The cysteine desulfurase IscS is a highly conserved master enzyme initiating sulfur transfer via persulfide to a range of acceptor proteins involved in Fe-S cluster assembly, tRNA modifications, and sulfur-containing cofactor biosynthesis. IscS is a highly conserved, widely distributed pyridoxal-5′-phosphate (PLP)-dependent enzyme, with 60% sequence identity between the enzyme from Escherichia coli and its human homolog, NFS1. It initiates intracellular sulfur trafficking, delivering the sulfur to several sulfur-accepting proteins such as IscU, ThiI, TusA, and MoaD/MoeB that commit the sulfur to different metabolic pathways, including iron-sulfur cluster assembly, thiamine and biotin synthesis, tRNA modifications, or molybdopterin biosynthesis. The small domain (residues 1–15 and 264–404) contains the critical active site cysteine Cys328.

As established previously, the IscS-IscU complex is also a heterotetramer. IscU binds near the C-terminus of IscS, forming a very elongated S-shaped heterotetrameric protein complex 150 Å long and 65 Å wide. The IscU is in its apo form, with no evidence of a bound Fe-S cluster. IscU is a two-layered α/β sandwich with a core three-stranded β-sheet and bundle of five α-helices. IscU makes contacts with helix α8IscS (Glu309-Ala316), helical turn α10IscS (Glu347), the end of helix α11IscS, and the C-terminal helix α12IscS (Arg379-Lys391). The bound IscU projects its most conserved surface containing three conserved cysteines toward the IscS loop that carries Cys328. The distance between the modeled Cys328IscS and any cysteine of IscU in our structure is greater than ∼12 Å, implying that a conformational change must accompany sulfur transfer. Each IscU molecule interacts with only one subunit of the IscS dimer and, based on its orientation in the complex, would be expected to accept sulfur from the same subunit to which it is bound. Since most regions of IscS show no differences in the various crystal structures, either alone or complexed with acceptor proteins, and in view of the high flexibility/disorder of the Cys328 loop, we postulate that it is this loop that bends closer toward IscU in order to effect sulfur transfer.

> GSAYSEKVIDHYENPRNVGSFDNNDENVGSGMVGAPACGDVMKLQIKVNDEGIIEDARFKTYGCGSAIASSSLVTEWVKGKSLDEAQAIKNTDIAEELELPPVKIHCSILAEDAIKAAIADYKSKREAK;> MGSSHHHHHHGSMYGVYRAMKLPIYLDYSATTPVDPRVAEKMMQFMTMDGTFGNPASRSHRFGWQAEEAVDIARNQIADLVGADPREIVFTSGATESDNLAIKGAANFYQKKGKHIITSKTEHKAVLDTCRQLEREGFEVTYLAPQRNGIIDLKELEAAMRDDTILVSIMHVNNEIGVVQDIAAIGEMCRARGIIYHVDATQSVGKLPIDLSQLKVDLMSFSGHKIYGPKGIGALYVRRKPRVRIEAQMHGGGHERGMRSGTLPVHQIVGMGEAYRIAKEEMATEMERLRGLRNRLWNGIKDIEEVYLNGDLEHGAPNILNVSFNYVEGESLIMALKDLAVSSGSACTSASLEPSYVLRALGLNDELAHSSIRFSLGRFTTEEEIDYTIELVRKSIGRLRDLSPLWEMYKQGVDLNSIEWAHH> XI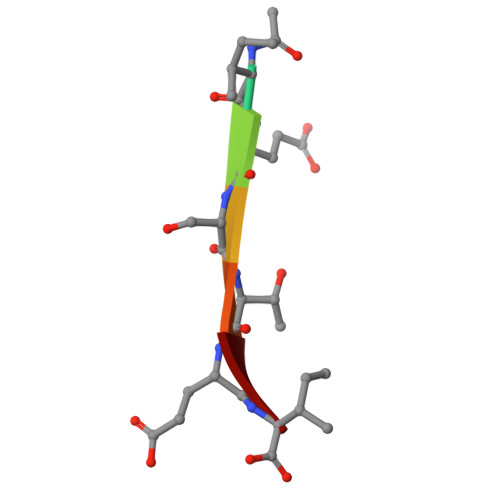ESTEI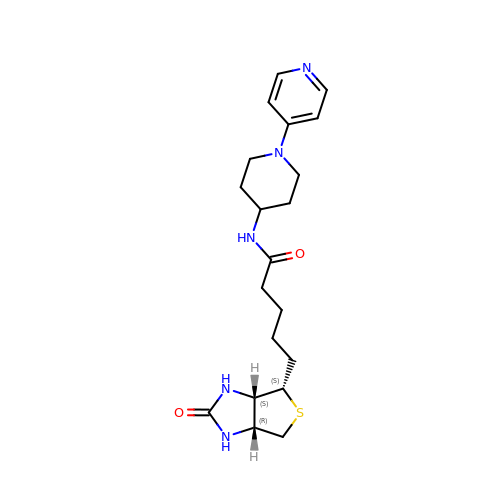5-[(3~{a}~{S},4~{S},6~{a}~{R})-2-oxidanylidene-1,3,3~{a},4,6,6~{a}-hexahydrothieno[3,4-d]imidazol-4-yl]-~{N}-(1-pyridin-4-ylpiperidin-4-yl)pentanamide | C20 H29 N5 O2 S | GEHXEZPHNHPYOB-LNLFQRSKSA-N> MKMTSIQQRAELHRQIWQIANDVRGSVDGWDFKQYVLGALFYRFISENFSSYIEAGDDSICYAKLDDSVITDDIKDDAIKTKGYFIYPSQLFCNVAAKANTNDRLNADLNSIFVAIESSAYGYPSEADIKGLFADFDTTSNRLGNTVKDKNARLAAVLKGVEGLKLGDFNEHQIDLFGDAYEFLISNYAANAGKSGGEFFTPQHVSKLIAQLAMHGQTHVNKIYDPAAGSGSLLLQAKKQFDNHIIEEGFFGQEINHTTYNLARMNMFLHNINYDKFDIKLGNTLTEPHFRDEKPFDAIV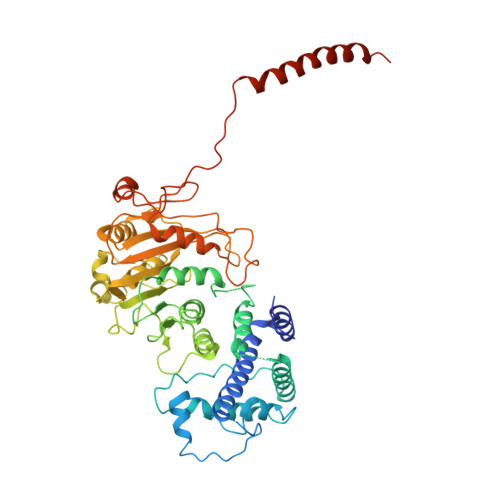SNPPYSVKWIGSDDPTLINDERFAPAGVLAPKSKADFAFVLHALNYLSAKGRAAIVCFPGIFYRGGAEQKIRQYLVDNNYVETVISLAPNLFFGTTIAVNILVLSKHKTDTNVQFIDASELFKKETNNNILTDAHIEQIMQVFASKEDVAHLAKSVAFETVVANDYNLSVSSYVEAKDNREIIDIAELNAELKTTVSKIDQLRKDIDAIVAEIEGCEVQK Biogenesis involves the de novo synthesis of a Fe/S cluster on the scaffold protein ISCU, trafficking of the cluster via transient association to various targeting factors, and finally cluster insertion into specific recipient apoproteins. A critical initial step in Fe/S cluster synthesis is the supply of sulfur by the cysteine desulfurase NFS1. Here, we report crystal and solution structures of human NFS1 in association with ISD11-ACP, ISCU, FDX2, and FXN, together forming the ‘core ISC complex’. We show that eukaryote-specific ISD11 binds to NFS1 distal from the desulfurase active site and does not directly participate in catalysis.

Crystals obtained from purifications in the presence of ethylenediaminetetraacetic acid (EDTA) (termed (NIAU)2) did not contain divalent ions and diffracted to 3.15 Å, while those from purifications without EDTA contained a Zn ion bound between NFS1 and ISCU ((NIAU-Zn)2) and diffracted to 3.3 Å. Two ISCU monomers are bound at opposite tips of the NFS1 dimer. The NFS1 residues binding ISCU include the C-terminal Tyr360-Lys371, His403, Arg432-Thr455, and the tip of the Cys-loop. In particular, the C-terminal Met436-Thr455 wrap tightly around ISCU. Conspicuously, ISCU binding to the C-terminal segment of NFS1 rigidifies the disordered regions through a ‘domino effect’ and re-creates the ‘standard’ dimer interface. ISCU attaches to NFS1 with the end that contains potential ligands for Fe/S cluster binding, Cys44, Asp46, Cys70, His112, and Cys113. In (NIAU)2 this ISCU metal binding site is empty; the conserved ‘Ala-loop’ (Ala41-Pro42-Ala43-Cys44) of ISCU contacts Glu399 and Trp454 side-chains of NFS1, with Cys44ISCU facing away from the Fe/S cluster binding site. The Cys-loop of NFS1 extends towards ISCU, but its tip (Cys381-Ser385) is disordered and not visible in the electron density. We conclude that ISCU binding dynamically changes the NFS1 structure thereby facilitating sulfur transfer from NFS1.

>[2x]MGSSLRPLYMDVQATTPLDPRVLDAMLPYLINYYGNPHSRTHAYGWESEAAMERARQQVASLIGADPREIIFTSGATESNNIAIKGVARFYRSRKKHLITTQTEHKCVLDSCRSLEAEGFQVTYLPVQKSGIIDLKELEAAIQPDTSLVSVMTVNNEIGVKQPIAEIGRICSSRKVYFHTDAAQAVGKIPLDVNDMKIDLMSISGHKIYGPKGVGAIYIRRRPRVRVEALQSGGGQERGMRSGTVPTPLVVGLGAACEVAQQEMEYDHKRISKLSERLIQNIMKSLPDVVMNGDPKHHYPGCINLSFAYVEGESLLMALKDVALSSGSACTSASLEPSYVLRAIGTDEDLAHSSIRFGIGRFTTEEEVDYTVEKCIQHVKRLREMSPLWEMVQDGIDLKSIKWTQH;>[2x]MAASSRAQVLALYRAMLRESKRFSAYNYRTYAVRRIRDAFRENKNVKDPVEIQTLVNKAKRDLGVIRRQVHIGQLYSTDKLIIENRDMPRT;>[2x]STIEERVKKIIGEQLGVKQEEVTNNASFVEDLGADSLDTVELVMALEEEFDTEIPDEEAEKITTVQAAIDYINGHQA;>MVLIDMSVDLSTQVVDHYENPRNVGSLDKTSKNVGTGLVGAPACGDVMKLQIQVDEKGKIVDARFKTFGCGSAIASSSLATEWVKGKTVEEALTIKNTDIAKELCLPPVKLHCSILAEDAIKAALADYKLKQEPKKGEAEKKLEHHHHHH[2x]>GDAGYISFKANGGVRLADEEHLASLLVDTNDYKGLQRAAADLQTDMQRVTGKLPTLHSQLKDAGRHAVIIGSVGRSGLIQLLVEQNKLNVADIEGQWEAYKLVVVDKPFPNIEKALVIAGSDMRGAIFGVYDLSQQIGVSPWYWWADVPVQPQSKLYVRGDTHIVEQPKVQYRGIFLNDEAPALTNWVHANYGNYNSQFYTQVFELLLRLKANFLWPAMWNNSFSVDDPLNPVLANEYGIVMSTSHHEPMMRAHKEWHGMGRWDFTTNADALKQFWREGVERNSPYENIITMAMRGDGDEAMSEDANVELLEQIVEAQRNIIAEVFEPKGKQVTEVPQVWCLYKEVQDYYEKGMRVPDDITLLWADDNWGNIRRLPTAEERKRSGGAGVYYHFDYVGGPRSYRWINTTPLAKIWEQMHLAYKYEANKIWIVNVGDLKPMEAPIEYFLEMAWNPEQWPKERITQFAELWAEREFGPTYAKEIAQLVQDYTQHNGRRKPELQEAKTYSLLNYDEAARIEQQLTDMESRAETLFNKIPANQRDAYYQLVMHPVLASATVTKMYIAQARNRLYAKQGRPIANSYGQQVKELFEKDAALTKRYHSINNGKWNHFMSQPHIGYTHWNNPEDNIMPVVSVVSKGNNADMGVAVEGMEPAWPTQDVAFALPTFTPYGKQTKILTVFNKGVKPLKFSVSSGAAWLKVSASSGEITHQEMQIQVSIDWAKLPLGIHESNVTIKGPSWVAANIKVTANKPAKVIPLKKLTGFVEADGYISFDAAATTHSKAVDGFEWQEIPAHGRTHS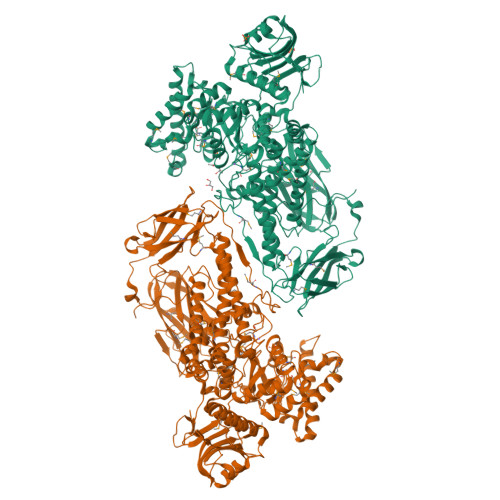SMSVYPIRDASFAAPANASANTAPQMHYSITLLTAGEVTVEGLFAPTWPIHPERGLRYAIAFDDQPPQIVDVLAGNSHKVWQESVRTGVRRASSKHTLTAGTHTMKVWAIDPAVTVQKWIIDTGELKPSYLGPTPSPRGGKH[2x]>[4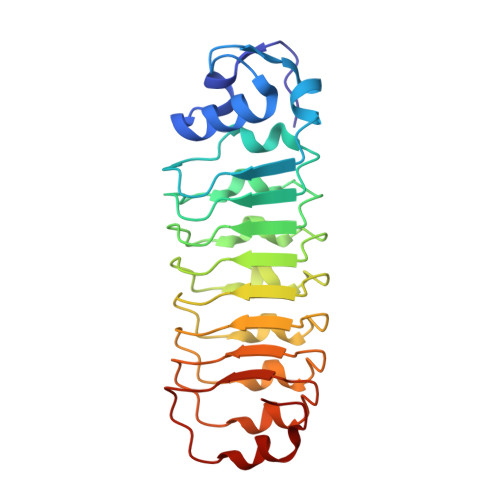x]ETITVSTPIKQIFPDDAFAETIKANLKKKSVTDAVTQNELNSIDQIIANNSDIKSVQGIQYLPNLKTLKLSNNKITDISALKQLNNLGWLDLSNNGITDISALKNLASLHTLDLSNNGITDISALKNLDNLHTLDLSNNGITDISALKNLDNLHTLDLSNNGITDISALKNLTSLHTLDLSNNGITDISALKNLDNLETLDLRNNGITDKSALKNLNNLK> MTHFSTVKRVIALAGAGAMLFSVAACGGVTASDGGKTTLKFAAFEGGYGADMYKEVVAAYEKLNPDVKIELTTSKKIEDEITPGMKAGNYPDIVELGQGSTSGLTETLLKDKAIEDVTDVLDMKVPGENKTVKDKLVDGVIGLYTNPYGGDKTYLMPMYYSPSGLVYNKTLLEQNGWKMPTTWDEMFKLGDEAKAKGISLFTYPTAGYFDAFFNALLADIGGDQFYQDVMTYKKDVWKTDEAKEALETTYKLVTEYLNPDTVGYANAQDFTKNQQSILDGKSLFMPNGTWIVNEMKDAPRTSGFEWGFAPVPTVKNGGTRYINTTIEAVWIPAKAKNKEAAKKFMAYLYSDEAASIFAKTGAIQPIKGNTDDLASDMKVFYDAYNEDNVKAVAGSFSATATVEGKN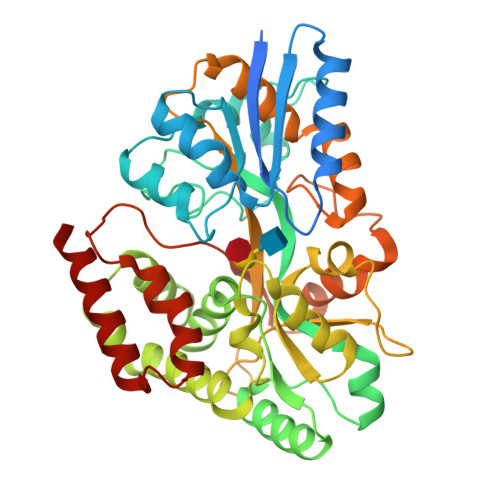IKDDLYNAVDSVASGKTTLQQWQDKLNETSNALNAAAKQ>NGPSPNLPPGFDFTDPAIYAERLPVAEFAELRSAAPIWWNGQDPGKGGGFHDGGFWAITKLNDVKEISRHSDVFSSYENGVIPRFKNDIAREDIEVQRFVMLNMDAPHHTRLRKIISRGFTPRAVGRLHDELQERAQKIAAEAAAAGSGDFVEQVSCELPLQAIAGLLGVPQEDRGKLFHWSNEMTGNEDPEYAHIDPKASSAELIGYAMKMAEEKAKNPADDIVTQLIQADIDGEKLSDDEFGFFVVMLAVAGNETTRNSITQGMMAFAEHPDQWELYKKVRPETAADEIVRWATPVTAFQRTALRDYELSGVQIKKGQRVVMFYRSANFDEEVFQDPFTF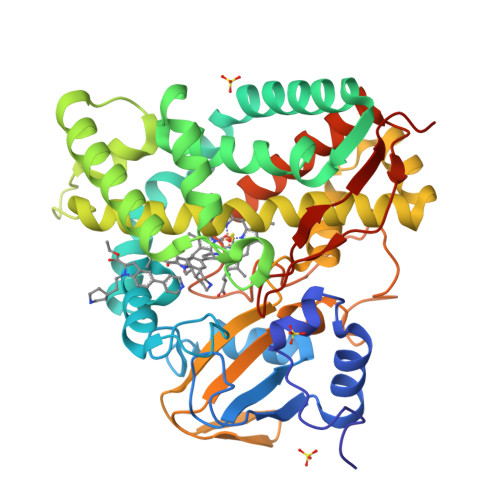NILRNPNPHVGFGGTGAHYCIGANLARMTINLIFNAVADHMPDLKPISAPERLRSGWLNGIKHWQVDYTGRCPVAH[3x]> XCAIDQDFLDAAGILENEAIDIWNVTNGKRFSTYAIAAERGSRIISVQGAAAHCASVGDIVIIASFVTMPDEEARTWRPNVAYFE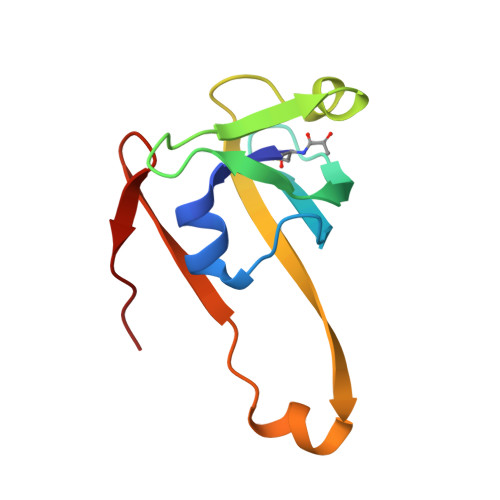GDNEMKRTAK> QYSPNTQQGRTSIVHLFEWRWVDIALECERYLAPKGFGGVQVSPPNENVAIYNPFRPWWERYQPVSYKLCTRSGNEDEFRNMVTRCNNVGVRIYVDAVINHMCGNAVSAGTSSTCGS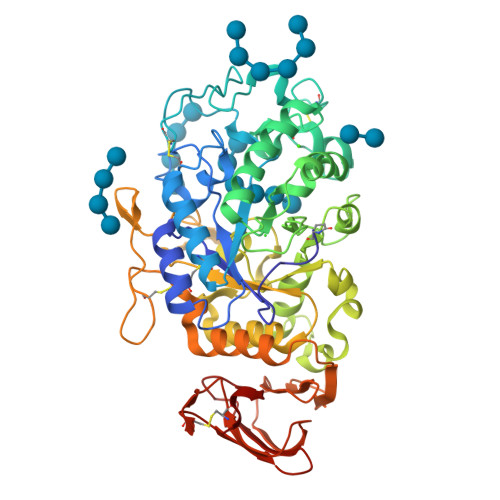YFNPGSRDFPAVPYSGWDFNDGKCKTGSGDIENYNDATQVRDCRLTGLLDLALEKDYVRSKIAEYMNHLIDIGVAGFRLDASKHMWPGDIKAILDKLHNLNSNWFPAGSKPFIYQEVIDLGGEPIKSSDYFGNGRVTEFKYGAKLGTVIRKWNGEKMSYLKNWGEGWGFVPSDRALVFVDNHNNQRGHGAGGASILTFWDARLYKMAVGFMLAHPYGFTRVMSSYRWPRQFQNGNDVNDWVGPPNNNGVIKEVTINPDTTCGNDWVCEHRWRQIRNMVIFRNVVDGQPFTNWYDNGSNQVAFGRGNRGFIVFNNDDWSFSLTLQTGLPAGTYCDVISGDKINGNCTGIKIYVSDDGKAHFSISNSAEDPFIAIHAESKL>[2x]MKQVCVLGNGQLGRMLRQAGEPLGIAVWPVGLDAEPAAVPFQQSVITAEIERWPETALTRQLARHPAFVNRDVFPIIADRLTQKQLFDKLHLPTAPWQLLAERSEWPAVFDRLGELAIVKRRTGGYDGRGQWRLRANETEQLPAECYGECIVEQGINFSGEVSLVGARGFDGSTVFYPLTHNL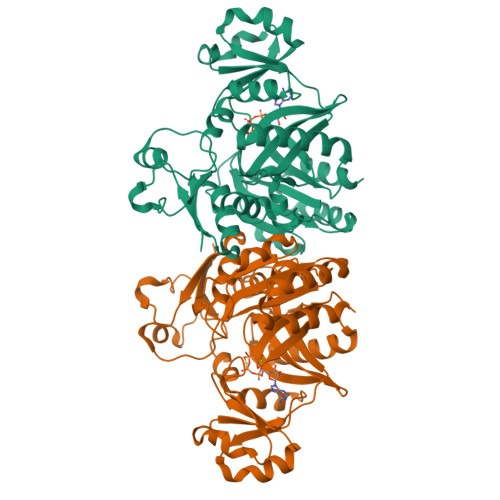HQDGILRTSVAFPQANAQQQARAEEMLSAIMQELGYVGVMAMECFVTPQGLLINELAPRVHNSGHWTQNGASISQFELHLRAITDLPLPQPVVNNPSVMINLIGSDVNYDWLKLPLVHLHWYDKEVRPGRKVGHLNLTDSDTSRLTATLEALIPLLPPEYASGVIWAQSKFG> GSHMGTRDDEYDYLFKVVLIGDSGVGKSNLLSRFTRNEFNLESKSTIGVEFATRSIQVDGKTIKAQIWDTAGLERYRAITSAYYRGAVGALLVYDIAKHLTYENVERWLKELRDHADSNIVIMLVGNKSDLRHLRAVPTDEARAFAEKNGLSFIETSALDSTNVEAAFQTILTEIYRIVSQK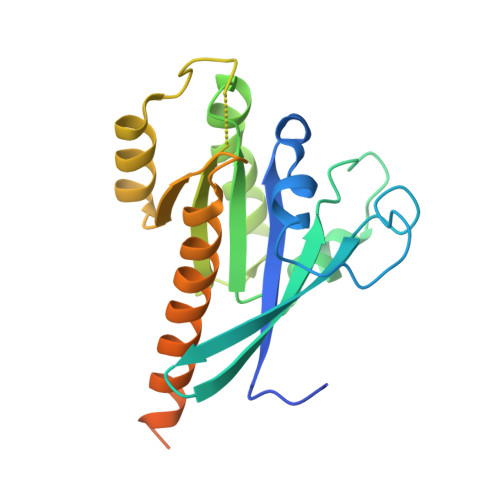QMSDRRENDMSPSNNVVPIHVPPTTENKPKVQCCQNI> MIERGKFRSLTLVNWNGFFARTFDLDELVTTLSGGNGAGKSTTMAAFVTALIPDLTLLHFRNTTEAGATSGSRDKGLHGKLRA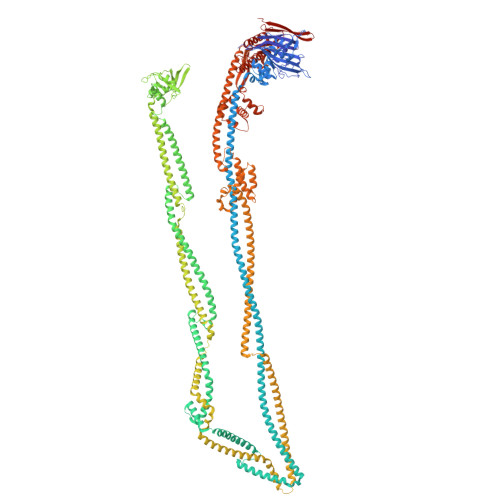GVCYSTLDVINSRHQRVVVGVRLQQVAGRDRKVDIKPFMIQGLPTAIQPTQLLTENVGERQARVLPLNELKDRLDEMEGVQFKQFNSITDYHAQMFDLGVIPKRLRSASDRSKFYRLIEASLYGGISSAITRSLRDYLLPENSGVRKAFQDMEAALRENRITLEAIRVTQSDRDLFKHLITEATSYVSADYMRHANERRTHLDEALALRGELFGSHKQLATEQYRHVEMARELAEQSGASSDLETDHQAASDHLNLVQTAMRQQEKIDRYQVDLEELSYRLEEQTDVVEEAGELQAEYEARTEATEQEVDELKSQLADYQQALDVQQTRAIQYQQALQALERARELCRLPDLSVDNAEEWLETFQAKEQQATEALLALEQKLSVADAAHNQFEQAYQLVKNIVGETSRSEAWQSARELLRDWPSQRHLADRVQPLRMRLSELEQRLNNQQNAERLLSEFCKRQGRQYQAEDLEALQNELEARQEALSLSVNEGGERRMEMRQELEQLKQKIQSLTARAPVWLAAQDTLNQLCEQSGETLASSNDVTEYMQQLLEREREATVERDEVAAQKRELEKQIERLSQPSGAEDSRMIALAERFGGVLLSEIYDDITIDDAPYFSALYGPARHGIVVPDLSLVRPHLETLEDCPEDLYLIEGDPQSFDDSVFNAEEQTNAVLVKSSDRQWRYSRYPELPLFGRAARENRLEALNLERDALAERYATLSFDVQKIQRAHQAFSQFVGKHLSVAFDTDPEAEIRELRQRHTELEREVSRFEDQTQQQRQQYAQAKESLTTLNRLIPQVTLLLDETLIDRVEEVREEMDEAQEAARFLQQHGSALTKLEPMVAVLQSDPQQHEQLQQDYETAKHSQHQAKQQAFALVEIVQRRVHFSYSDSAGMLSENADLNDKLRQRLEHAESDRSRAREQLRQQQAQYSQFNQVLASLKSSYETKQDMLKELLQEMKDIGVQADANAEMRARERRDRLHEALSVNRSRVNQLEKQIAFCEAEMENVQKKLRKLERDYYQIREQVVSAKAGWCAVMRMVKDNGVERRLHRRELAYMEGGALRSMSDKALGALRLAVADNEHLRDALRLSEDPKRPERKVQFFIAVYQHLRERIRQDIIRTDDPVDAIEQMEIELARLTEELTAREQKLAISSKSVANIIRKTIQREQNRIRMLNQGLQAVSFGQVRGVRLNVNVRESHAILLDVLSEQQEQHQDLFNSQRLTFSEAMAKLYQRLNPQVDMGQRLPQTIGEELLDYRNYLELDVEVNRGSDGWLKAESGALSTGEAIGTGMSILVMVVQSWEEESRRLRGKDISPCRLLFLDQAARLDAKSIATLFELCERLQMQLIIAAPENISPEKGTTYKLVRKVFKNHEHVHVVGLRGFGQDAPATQLISDVTA N-acetylglucosaminono-1,5-lactone 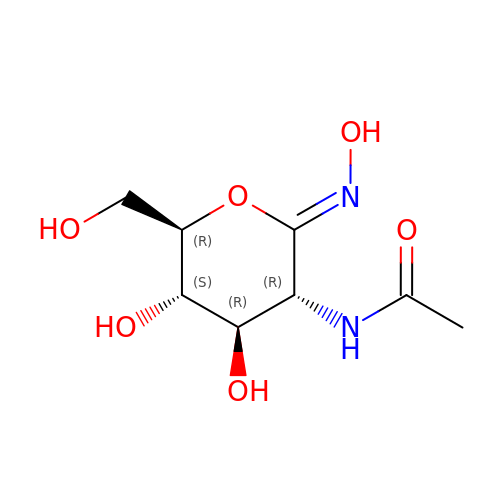(Z)-oxime | C8 H14 N2 O6 | NJBKCLCEXIDHDR-OANDGCGGSA-N>[2x]MELKHSISDYTEAEFLQLVTTICNADTS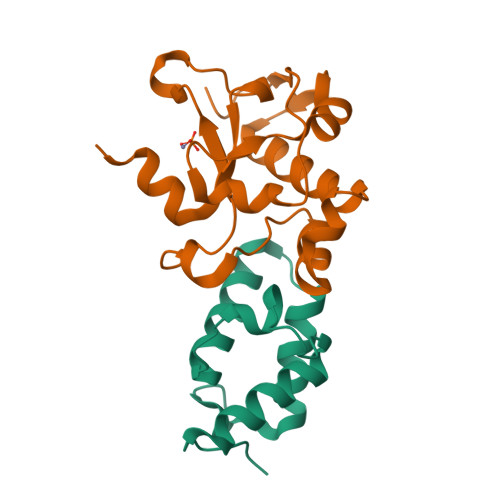SEEELVKLVTHFEEMTEHPSGSALIYYPKEGDDDSPSGIVNTVKQWRAANGKSGFKQG;>MESKRNKPGKATGKGKPVGDKWLDDAGKDSGAPIPDRIADKLRDKEFKSFDDFRKAVWEEVSKDPELSKNLNPSNKSSVSKGYSPFTPKNQQVGGRKVYELHHDKPISQGGEVYDMDNIRVTTPKRHIDIHRGK[2x]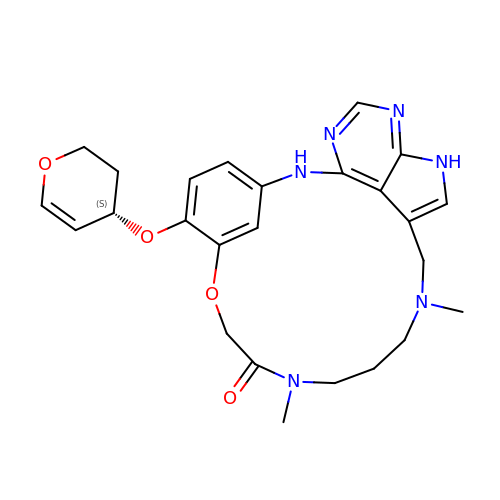11,15-Dimethyl-6-(oxan-4-yloxy)-8-oxa-2,11,15,19,21,23-hexazatetracyclo[15.6.1.13,7.020,24]pentacosa-1(23),3(25),4,6,17,20(24),21-heptaen-10-one | C25 H30 N6 O4 | HPBBITAJZLZSRK-LJQANCHMSA-N> MKTVVFAYHDMGCLGIEALLAAGYEISAIFTHTDNPGEKAFYGSVARLAAERGIPVYAPDNVNHPLWVERIAQLSPDVIFSFYYRHLIYDEILQLAPAGAFNLHGSLLPKYRGRAPLNWVLVNGETETGVTLHRMVKRADAGAIVAQLRIAIAPDDIAITLHHKLCHAARQLLEQTLPAIKHGNILEIAQRENEATCFGRRTPDDSFLEWHKPASVLHNMVRAVADPWPGAFSYVGNQKFTVWSSRVHPHASKAQPGSVISVAPLLIACGDGALEIVTGQAGDGITMQ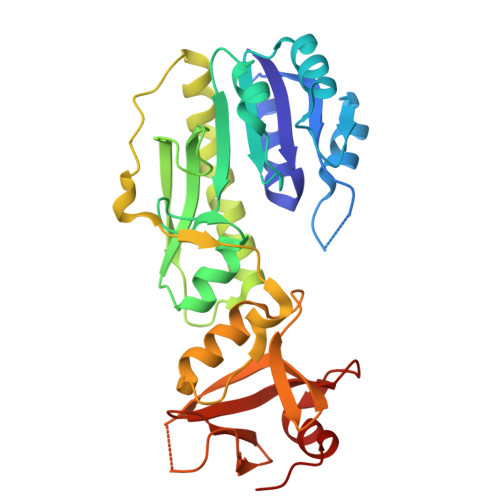GSQLAQTLGLVQ> SNAMIFPKQYPIINFTTAGATVQSYTNFIRAVRGRLTTGADVRHEIPVLPNRVGLPINQRFILVELSNHAELSVTLALDVTNAYVVGYRAGNSAYFFHPDNQEDAEAITHLFTDVQNRYTFAFGGNYDRLEQLAGNLRENIELGNGPLEEAISALYYYSTGGTQLPTLARSFIICIQMISEAARFQYIEGEMRTRIRYNRRSAPDPSVITLENSWGRLSTAIQESNQGAFASPIQLQRRNGSKFSVYDVSILIPIIALMVYRCAPPPSSQF

Ricin contains an active A subunit (RTA) and a B subunit (RTB), which promotes retrograde transport into the endoplasmic reticulum (ER). RTA and Stx2A1 are ribosome inactivating proteins (RIPs), which remove a highly conserved adenine base (A4324 in rat) from the sarcin/ricin loop (SRL) of the 28S rRNA, leading to the inhibition of translation, ribotoxic stress, and apoptosis. We showed that RTA is recruited to the SRL by binding first to a conserved sequence at the C-terminal domain (CTD) of ribosomal P-stalk proteins. The X-ray crystal structure analysis showed that RTA binds the last six amino acids of P11 in a hydrophobic pocket at its CTD.

The RTA-RU-NT-202, RTA-RU-NT-165, and RTA-RU-NT-192 structures were all determined at 1.8 Å. The RTA-RU-NT-165 and RTA-RU-NT-192 structures were determined in the monoclinic P21 space group with the RTA-RU-NT-202 complex structures solved in the orthorhombic P212121 space group. Although all three inhibitors bound similarly to the P-stalk pocket, RU-NT-202 adopted a notably different orientation, rotating its carboxylate moiety 91° compared to RU-NT-192 and RU-NT-165. This shifted the thiophene carboxylate position in RU-NT-202 ∼2 Å away from Arg234, thereby precluding any interaction with this residue and potentially reducing binding affinity for RTA. In contrast, the thiophene carboxylate in RU-NT-202 only interacted with Arg235, forming a salt bridge with the side chain and a hydrogen bond with the main chain of Arg235. The fluorine atom of the fluorobenzene ring in RU-NT-202 uniquely interacted with Val242 in RTA, while making closer contacts with Ile247 and Leu248. The fluorine atom in the fluorobenzene ring of RU-NT-202 interacted specifically with several nonpolar residues lining the P-stalk pocket, causing a shift in the position of RU-NT-202's benzene ring within the pocket compared to RU-NT-192, repositioning the thiophene ring and carboxylate group of RU-NT-202 away from Arg234. The RU-NT-202 carboxylate also rotated by 91° relative to RU-NT-192, further distancing the carboxylate of RU-NT-202 from Arg234. Consequently, the carboxylate group of RU-NT-202 did not interact noncovalently with Arg234, potentially reducing the binding affinity and inhibitory potency compared to RU-NT-192. Furthermore, the relatively altered position of the fluorobenzene ring in RU-NT-202 prevented hydrophobic contacts with Leu207, which may have further diminished the inhibitory function.>[4x]MLYHLFVNNQVKLQNDFKPE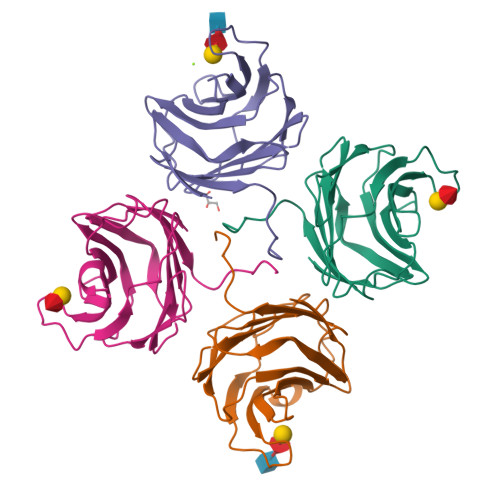SVAAIRSSAFNSKGGTTVFNFLSAGENILLHISIRPGENVIVFNSRLKNGAWGPEERIPYAEKFRPPNPSITVIDHGDRFQIRFDYGTSIYYNKRIKENAAAIAYNAENSLFSSPVTVDVHGLLPPLPPA> AQVINTNSLSLLTQNNLNKSQSALGTAIERLSSGLRINSAKDDAAGQAIANRFTANIKGLTQASRNANDGISIAQTTEGALNEINNNLQRVRELAVQSANSTNSQSDLDSIQAEITQRLNEIDRVSGQTQFNGVKVLAQDNTLTIQVGANDGETIDIDLKQINSQTLGLDTLNVQQKYKVSDTAATVTGYADTTIALDNSTFKASATGLGGTDQKIDGDLKFDDTTGKYYAKVTVTGGTGKDGYYEVSVDKTNGEVTLAGGATSPLTGGLPATATEDVKNVQVANADLTEAKAALTAAGVTGTASVVKMSYTDNNGKTIDGGLAVKVGDDYYSATQNKDGSISINTTKYTADDGTSKTALNKLGGADGKTEVVSIGGKTYAASKAEGHNFKAQPDLAEAAATTTENPLQKIDAALAQVDTLRSDLAAVQNRFNSAITNLGNTVNNLTSARSRIEDSDYATEVSNMSRA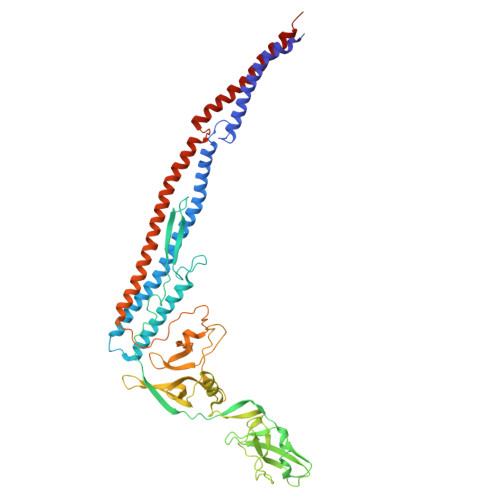QILQQAGTSVLAQANQVPQNVLSLLR>SAQTIEATSVKQLADAGVRVGDTLRISGTGMCNIRTSGTWSAKTNSPFLPFDCSQIIWNDARSLPLPESELVNKATALTEAVNRQLHPKPEDESRVSASLRSAIQKSGMVLLDDFGDIVLKTADLCSAKDDCVRLKNALVNLGNSKDWDALVKRANAGKLDGVNVLLRPVSAESLDNLVATSTAPFITHETARAAQSLNSPAPGGFLIVSDEGSD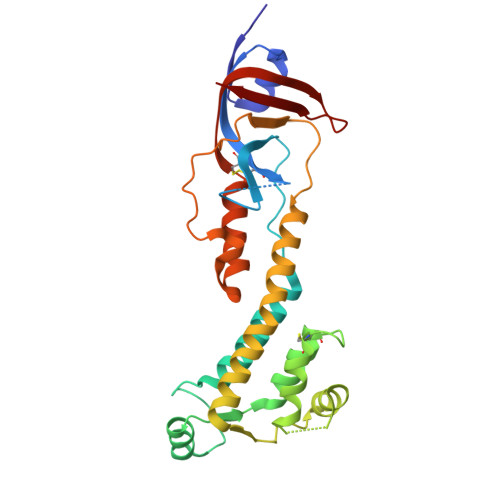FVDQPWPSASLYDYPPQEQWNAFQKLAQMLMHTPFNAEGIVTKIFTDANGTQHIGLHPI[2x]Here, we functionally characterize a transcriptional regulator, BrxR, encoded within a recently described phage defence island from a multidrug resistant plasmid of the emerging pathogen Escherichia fergusonii. Using a combination of reporters and electrophoretic mobility shift assays, we discovered that BrxR acts as a repressor. BrxR comprises an N-terminal winged-HTH domain (residues 1–94), followed by a WYL-domain (so called due to a previous analysis of conserved amino acids), which has been implicated as a potential ligand-binding domain with a role in phage defence (residues 120–190), and a C-terminal dimerization domain (residues 200–295).

We solved the structure of BrxR by X-ray crystallography, to 2.15 Å. The asymmetric unit contained four BrxR dimers, supporting our previous SEC data that indicated BrxR is a dimer in solution. The wHTH domains are exchanged between the protomers, such that upon exiting the wHTH the protein fold crosses to the other side of the dimer, to the WYL-domain. The WYL-domains do not appear to directly interact, but the C-terminal dimerization domains extend across like two left hands shaking, interacting through the opposing C-terminal domain through the palms, and with the opposing WYL-domain through an α-helix at the utmost tip of the protomeric dimerization domain (residues 202–232). The wHTH domains are spaced ∼25 Å apart in the BrxR dimer, indicating additional movement is required to optimize the positions for interaction with the major grooves of target DNA. Two sulphate molecules are bound within each WYL-domain. Nevertheless, the position of the two sulphates corresponds to a solvent-exposed basic patch formed by each BrxR protomer. Detailed examination of the sulphate binding site in BrxREfer shows an abundance of polar groups that have captured the sulphate ions and could theoretically recognize other small molecule ligands. These residues are found within the core β-strands but also the conserved loops, such as S143, S145 and S146 on the RT loop; K173 and H174 on the distal loop; and R184 on the 310 α-helix. We propose that ligand-binding at the WYL-domain basic patch could induce conformational changes to BrxREfer that relieve transcriptional repression.

>MQDNTGLEELSQAQRERLAHIDFTLLFKGEAGRSYLTERFSVAPSVATQDFARYKALAPNNVMYDEKRRVHLKTSTFQPLFDYDIVRTLATISQGFGDGFLGKVRPPMACEAPFHLNKPKLEVVAAISEAIHKRAVINIEYTSLSSGHGSRQIVPHTLIDNGLRWHVRAFDRKHREFRDFVLTRISEVELLEDKVNDEVETLQWDKQWNRIVELELIPHPKLAHPEAVLIDYAMENNRLRVEIRAAFAGYLLRLWNIDCSKNSKSNGREFHLALKNPEALYGVDNAALAPGYSES[8x]> MKTDGEFVSEHLMELITQQNLTINRVATLAGLNQSTVNAMFEGRSKRPTITTIRKVCGTLGISVHDFFDFPP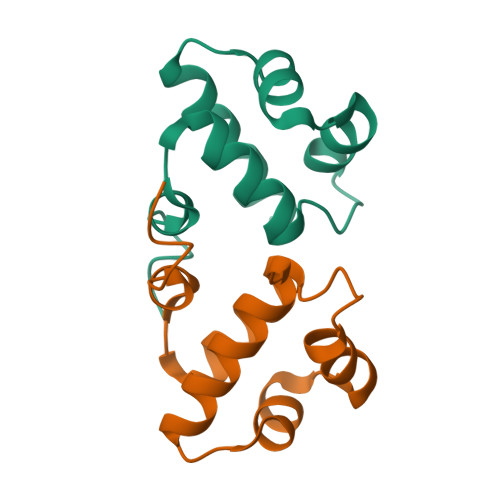YNEVEK>[3x]AMGSPIFGYSNTQQSQRVVTADNLMYLRSGFAIDAIGTTVNNLV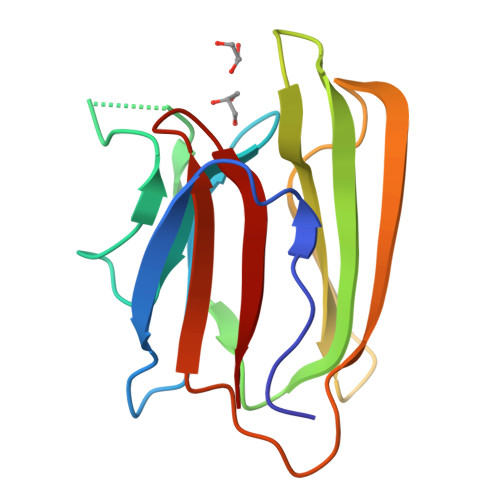GGPVQGTNGGVLRAPIALDQLQSVEVTSGLYNWGGYHIVAIKFTMKDGSSVLLGSTHYASNKKVETYTVPQGKRIKQINVWTGGWLVEGFQFVY The spliceosomal assembly, activation, catalysis and disassembly cycle is driven and controlled by eight highly conserved superfamily 2 RNA-dependent NTPases/RNA helicases and a single G protein, Snu114 (7,8). Snu114 bears striking resemblance to the prokaryotic/eukaryotic ribosomal translocases EF-G/eEF2, exhibiting the same five-domain arrangement preceded by a Snu114-specific, ca. 125 residue, acidic N-terminal region. A prime candidate for such functions is the Prp8 protein, which forms a salt-stable complex with Snu114 (15), extensively interacts with Snu114 G and G’ domains in structures of spliceosomal complexes and is generally considered a master regulator of the spliceosome. Still, this activity could be reliably quantified and we unequivocally showed that it is completely abrogated in the presence of Prp8SBR. The latter observation formally establishes Prp8 as a GTPase-inhibiting protein, and thus to the best of our knowledge as the first GTPase-regulatory factor, of Snu114.

Based on these observations, we prepared a recombinant Snu11472-1008–Prp8SBR complex by co-production of Snu11472-1008 and Prp8SBR in insect cells, and determined its crystal structure at 3.1 Å resolution. Crystals contained two independent copies of the Snu11472-1008–Prp8SBR complex, which were virtually identical (root-mean-square deviation [rmsd] of 0.66 Å for 997 pairs of Cα atoms). Snu11472-1008 contains five EF-G/eEF2-like domains, i.e. G, G’, II, III, IV and V, with the G’ domain inserted into the G domain, and domain V intervening between the IVa and IVb sub-domains. It adopts a compact conformation, in which the N-terminal G and G’ domains form a globular head that is cradled in an array of domains II, III and V, and in which the split domain IV forms a pedestal at the bottom. Prp8SBR exhibits an extended, loosely twisted conformation that lacks a globular fold, suggesting that the fragment would be intrinsically disordered in isolation. Residues 402–410 stretches along the open side of the nucleotide-binding pocket and the following residues 411–471 form a long loop, previously referred to as the Prp8 lasso, which encircles a protruding region of the G’ domain. In the crystal structure of the isolated Snu11472-1008–Prp8SBR complex, the electron density clearly indicated that both Snu114 molecules in an asymmetric unit were bound to GTP and a metal ion, most likely Mg2+, although no nucleotide had been added during purification or crystallization. Similar to the situation in structures of spliceosomal complexes, H218 in the isolated Snu11472-1008–Prp8SBR complex is rotated away from the GTP γ-phosphate, hydrogen bonding with the hydroxyl group of Prp8SBR Y403. W402 of Prp8SBR lies on top of the Snu11472-1008 switch I region, helping to anchor the neighboring Prp8SBR Y403 in front of the nucleotide-binding pocket.

>MKEVEVLMETKNTQSPQTPLVEPVTERTKLQEHTIFTQLKKNIPKTRYNRDYMLSMANIPERIINVGVIGPLHSGKTSLMDLLVIDSHKRIPDMSKNVELGWKPLRYLDNLKQEIDRGLSIKLNGSTLLCTDLESKSRMINFLDAPGHVNFMDETAVALAASDLVLIVIDVVEGVTFVVEQLIKQSIKNNVAMCFVINKLDRLILDLKLPPMDAYLKLNHIIANINSFTKGNVFSPIDNNIIFASTKLGFTFTIKEFVSYYYAHSIPSSKIDDFTTRLWGSVYYHKGNFRTKPFENVEKYPTFVEFILIPLYKIFSYALSMEKDKLKNLLRSNFRVNLSQEALQYDPQPFLKHVLQLIFRQQTGLVDAITRCYQPFELFDNKTAHLSIPGKSTPEGTLWAHVLKTVDYGGAEWSLVRIYSGLLKRGDTVRILDTSQSESRQKRQLHDISKTETSNEDEDEDDETPSCEVEEIGLLGGRYVYPVHEAHKGQIVLIKGISSAYIKSATLYSVKSKEDMKQLKFFKPLDYITEAVFKIVLQPLLPRELPKLLDALNKISKYYPGVIIKVEESGEHVILGNGELYMDCLLYDLRASYAKIEIKISDPLTVFSESCSNESFASIPVSNSISRLGEENLPGLSISVAAEPMDSKMIQDLSRNTLGKGQNCLDIDGIMDNPRKLSKILRTEYGWDSLASRNVWSFYNGNVLINDTLPDEISPELLSKYKEQIIQGFYWAVKEGPLAEEPIYGVQYKLLSISVPSDVNIDVMKSQIIPLMKKACYVGLLTAIPILLEPIYEVDITVHAPLLPIVEELMKKRRGSRIYKTIKVAGTPLLEVRGQVPVIESAGFETDLRLSTNGLGMCQLYFWHKIWRKVPGDVLDKDAFIPKLKPAPINSLSRDFVMKTRRRKGISTGGFMSNDGPTLEKYISAELYAQLRENGLVPWSHPQFEK[2x];>[2x]MWSHPQFEKSTPLRDEVTDKNYYYLFDKKSFFNGKALNNAIPGGPKFEPLYPREEEEDYNEFNSIDRVIFRVPIRSEYKVAFPHLYNSRPRSVRIPWYNNPVSCIIQNDEEYDTPALFFDPSLNPIPHFIDNNSSLNVSNTKENGDFTLPEDFAPLLAEEEELILPNTKDAMSLYHSPFPFNRTKGKMVRAQDVALAKKWFLQHPDEEYPVKVKVSYQKLLKNYVLNELHPTLPTNHNKTKLLKSLKNTK> GPGHMTTLTRQDLNFGQVVADVLCEFLEVAVHLILYVREVYPVGIFQKRKKYNVPVQMSCHPELNQYIQDTLHCVKPLLEKNDVEKVVVVILDKEHRPVEKFVFEITQPPLLSISSDSLLSHVEQLLAAFILKISVCDAVLDHNPPGCTFTVLVHTREAATRNMEKIQVIKDFPWILADEQDVHMHDPRLIPLKTMTSDILKMQLYVEERAHKGS;> MWFPYDGSK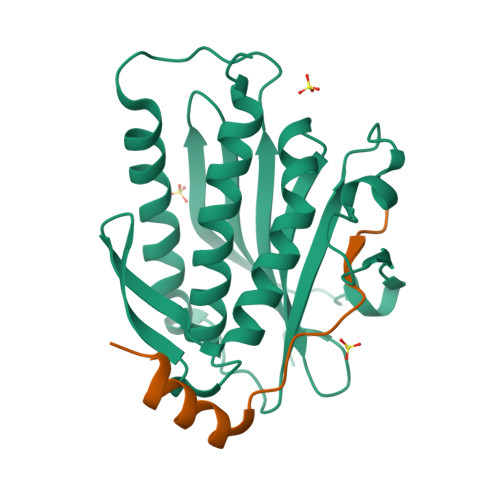LPLRPKRSPPVISEEAAEDVKQYLTI> AMADSELVAQWEKVQIKTFTKWVNMHLAKKGRKINDVTTDFKNGVELCALLEIIGETTIKCVTNPKMRIQMTENLDKALRFIQSRDVKLTGIGPTDIVDGNVKLTLGLVWTLILRFAISELSAEGLSAKQGLLLWCQKKCEPYPVKVENFSESFKDGKVFCALIHRHRPDLLDWETVGEDDRANLEKAFDVAEKELGIPKLLDVDDIVNMPRPDERSVM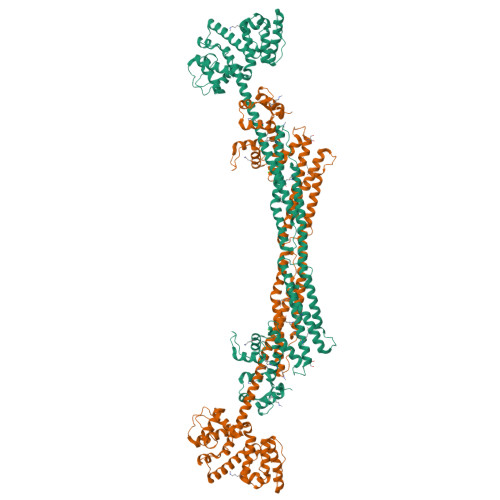TYVAALYKVFSSNDQVEKAGKRAGNFLDLLRATEGMVHDYEQRAQALKENIEAAINKMNGVEPSDEYHQVKEQINETKNYRKGDKRAFIKEQGDLATLFGQINSKLRGMKRPVYVAPEGLDPKSLEGYIANISEAERALRSKLNTAMRNCLIALRKAFADPANATDAKINEYRTFVTDETSEAPLEEQVATLKAKLEELKQVEAQLPPIEEAEKACGDANIEDNEYTDVSFDDLQFNYEQTVSMFEKKIVYIEAQINEASSGVTAEQMQEFKQSFDAFDGNHDGILDKLEFRSCLSSMGLIDIDFTGGEDAQYDAIYNNVTKGENGVSFDNYVQYMKEKNDENPSPEQLNEIFSTIAAGKDSITETDMQKAGMSAEQIEYVKANLPQKGDGYDYAAWVKTN> GAMDPMVTKEFLKIKLECSDMYAQKLIDEAQGDENKLYDLFIQK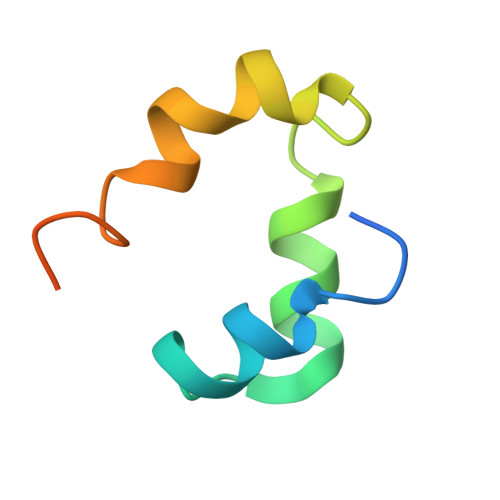LAERHTRPAIVEY>[2x]EPFSLPNLQTDEMSSSRWPNPLATLFADPNVAVAPQWQNGRCTLEGELLGTTPRNASWLNRFRGVSTAAVANQVLHLTLYEPDGSVFNPLSGAPAPEGFPDFTAQEYHLRAAGKVANTTGGGEIKSTDYTPALGGVKITAWDATGPSAGVEMTGQIESIGMENNTDFDVLPDYNGSAFDGSLNLAPPIVPLL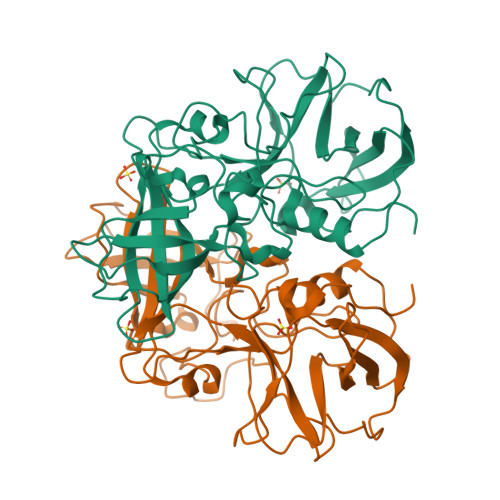PGETLLRFGTVPITTRRQSDPIRIISCALPQEWITWFLTHNFTALGDAALLRYRNQATGQLLFECKLYRSGFVVVNGVNVRTEFPMSGVFEFVSWVPNFFQLAPV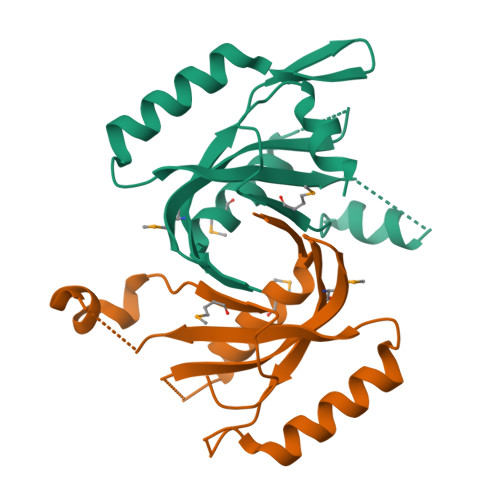>[2x]GSHMSVTISLHPLVIMNISEHWTRFRAQHGEPRQVYGALIGKQKGRNIEIMNSFELKTDVIGDETVINKDYYNKKEQQYKQVFSDLDFIGWYTTGDNPTADDIKIQRQIAAINECPIMLQLNPLSRSVDHLPLKLFESLID>AAVILESIFLKRSQQKKKTSPLNFKKRLFLLTVHKLSYYEYDFERGRRGSKKGSIDVEKITCVETVVPEKNPPPERQIPRRGEESSEMEQISIIERFPYPFQVVYDEGPLYVFSPTEELRKRWIHQLKNVIRYNSDLVQKYHPSFWIDGQYLCCSQTAKN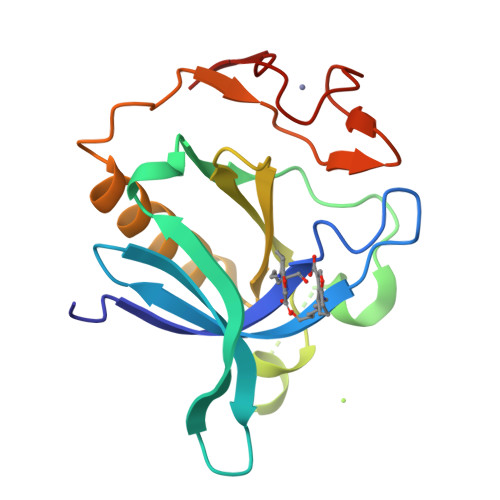AMGCQILEN[4x]Aspartate transcarbamoylase (ATC) catalyzes the second step of de novo pyrimidine synthesis, combining l-aspartate (l-ASP) and carbamoyl phosphate (CP) to form carbamoyl-aspartate (CP-ASP) and phosphate. Aspartate transcarbamoylase (ATC) has been suggested to be a promising target for antimalarial drug development. In depth structural analysis of the ATC catalytic cycle has been performed previously, which indicated that ATC exists in a low substrate affinity “T” state and a high substrate affinity “R” state. Here, we describe a series of small-molecule inhibitors of P. falciparum ATC with low nanomolar binding affinities that selectively bind to a previously unreported allosteric pocket, thereby inhibiting ATC activation.

Initially, we performed a 140-fragment structure-based screening experiment using a subset of an in-house multicomponent reaction (MCR)-compatible library and the availability of high-resolution crystals. As the smaller fragments used in our search will typically bind with lower affinities, resulting in weak electron density, pan dataset density analysis (PanDDa)15,16 was used to analyze the results of this fragment screening experiment. Fragments A, B, C, and D bind in a buried hydrophobic cavity formed by the α3 helix, α4 helix, and β1–3 sheets of the adjacent subunit. Enzymatic assays indicated an IC50 for these compounds of 10, 125, 150, and 145 μM, respectively.

>[3x]MFYINSKYKIDLDKIMTKMKNKSVINIDDVDDEELLAILYTSKQFEKILKNNEDSKYLENKVFCSVFLEPSTRTRCSFDAAILKLGSKVLNITDMNSTSFYKGETVEDAFKILSTYVDGIIYRDPSKKNVDIAVSSSSKPIINAGNGTGEHPTQSLLDFYTIHNYFPFILDRNINKKLNIAFVGDLKNGRTVHSLSKLLSRYNVSFNFVSCKSLNIPKDIVNTITYNLKKNNFYSDDSIKYFDNLEEGLEDVHIIYMTRIQKERFTDVDEYNQYKNAFILSNKTLENTRDDTKILHPLPRVNEIKVEVDSNPKSVYFTQAENGLYVRMALLYLIFSSTSSAWSHPQFEK methyl 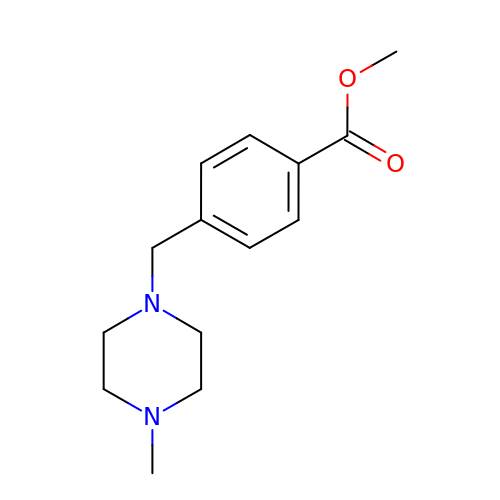4-[(4-methylpiperazin-1-yl)methyl]benzoate | C14 H20 N2 O2 | MEYCYFIWDAQKQK-UHFFFAOYSA-N>[4x]MGHHHHHHSGENLYFQGASMRTLLIRYILWRNDGDPSYYNDDFEKLMLLDELVDDSDVCTLIKNMRMTLSDGPLLDRLNQPVNNVEDVKRMIAIS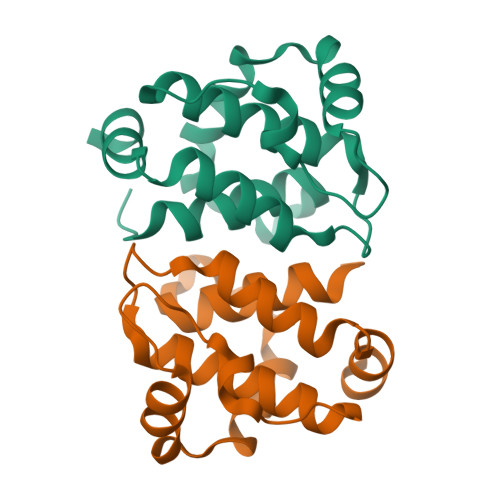AKVARDIGERPEIRWEESFTILFRMIETYFDDLMIDLYGEK>[6x]HSVAVIGAPFSQGQKRKGVEHGPAAIREAGLMKRLSSLGCHLKDFGDLSFTPVPKDDLYNNLIVNPRSVGLANQELAEVVSRAVSDGYSCVTLGGDHSLAIGTISGHARHCPDLCVVWVDAHADINTPLTTSSGNLHGQPVSFLLRELQDKVPQLPGFSWIKPCISSASIVYIGLRDVDPPEHFILK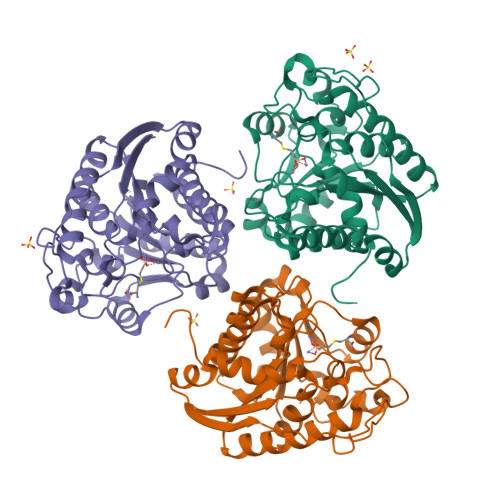NYDIQYFSMRDIDRLGIQKVMERTFDLLIGKRQRPIHLSFDIDAFDPTLAPATGTPVVGGLTYREGMYIAEEIHNTGLLSALDLVEVNPQLATSEEEAKTTANLAVDVIASSFGQTREG>[2x]GPTPEAPYASLTEIEHLVQSVCKSYRETCQLRLEDLLRQRSNIFSREEVTGYQRKSMWEMWERCAHHLTEAIQYVVEFAKRLSGFMELCQNDQIVLLKAGAMEVVLVRMCRAYNADNRTVFFEGKYGGMELFRALGCSELISSIFDFSHSLSALHFSEDEIALYTALVLINAHRPG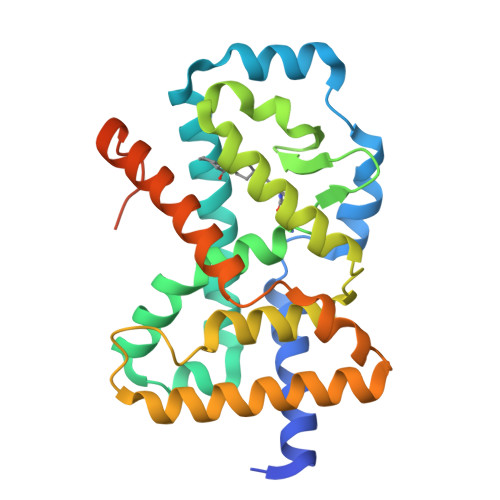LQEKRKVEQLQYNLELAFHHHLCKTHRQSILAKLPPKGKLRSLCSQHVERLQIFQHLHPIVVQAAFPPLYKELFSTETESPVGLSK> MNVGVNWSGQRELPCINQLFLTRDIDFVELLIDNFLTTDVDSIKAFLAGRPCAFHIMNSQFLHKDERELLAMAKIINKLIHSLQPIYISDHIGKFYHRGQALPQMLEVDYGLQTHSTIKKVKAWSSLLDGKLLLENYPSIFPQDMSQIDFFKRILEETYCGLLFDISNAFIAEVNIKQSRTSWFDLIKHCQHFHIAGFENAPDNQFLVDTHSQCIEEPV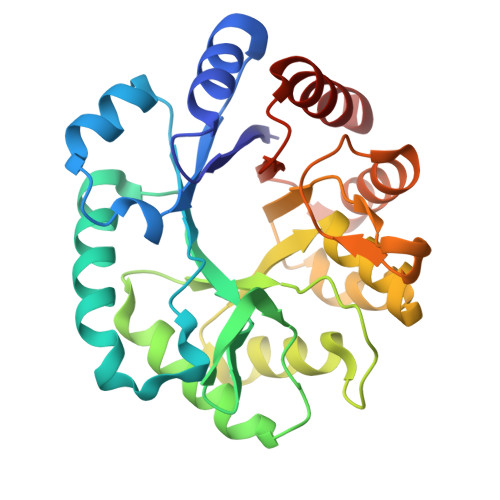LSFLQEVNNATSIATISVERDENFDVSDWALDIDNVRNRVS(5R)-5-hydroxy-3-methylfuran-2(5H)-one | 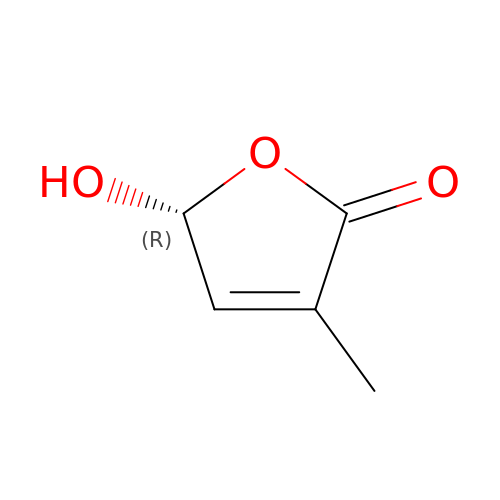C5 H6 O3 | HQIZYPQNJWENRT-SCSAIBSYSA-N>[4x]GSRRRAQHNEVERRRRDKINNWIVQLSKIIPDCNA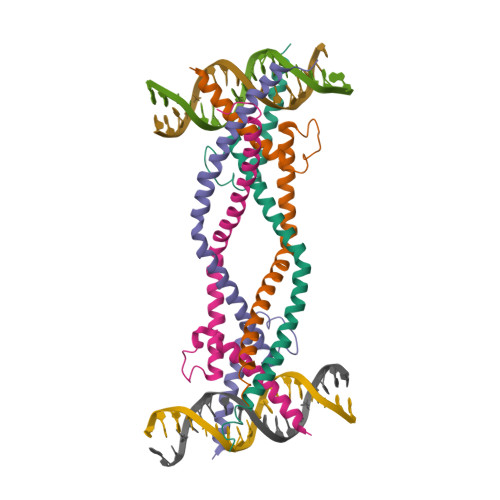DNSKTGASKGGILSKACDYIRELRQTNQRMQETFKEAERLQMDNELLRQQIEELKNENALLRAQLQQHNLEMVGEGTRQ>LRKVLISDSLDPCCRKILQDGGLQVVEKQNLSKEELIAELQDCEGLIVRSATKVTADVINAAEKLQVVGRAGTGVDNVDLEAATRKGILVMNTPNGNSLSAAELTCGMIMCLARQIPQATASMKDGKWERKKFMGTELNGKTLGILGLGRIGREVATRMQSFGMKTIGYDPIISPEVSASFGVQQLPLEEIWPLCDFITVHTPLLPSTTGLLNDNTFAQCKKGVRVVNCARGGIVDEGALLRALQSGQCAGAALDVFTEEPPRDRALVDHENVISCPHLGASTKEAQSRC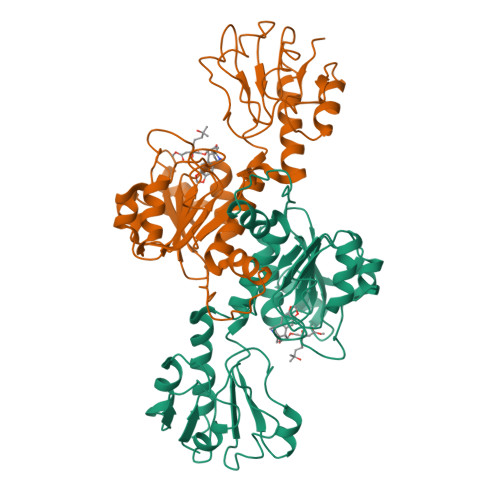GEEIAVQFVDMV[2x]> MSNVQTGAERMPHDLSHLGFLAGQIGRLITISTTPVIAGDSFEMDAVGALRLSPLRRGLAIDSTVDIFTFYVPHRHVYGEQWIKFMKDGVNAAPLPTVNTTGYIDHAAFLGTINPDTNKIPKHLFQGYLNIYNNYFKAPWMPDRTEANPNQLNEDDARYGFRCCHLKNIWTAPLPPETELSRQMTTSTTSIDIMGLQAAYANLHTDQERDYFMQRYRDVISSFGGKTSYDADNRPLLVMRSNFWASGYDVDGTDQTSLGQFSGRVQQTYKHSVPRFFVPEHGTMFTLALVRFPPTATKEIQYLNAKGALTYTDIAGD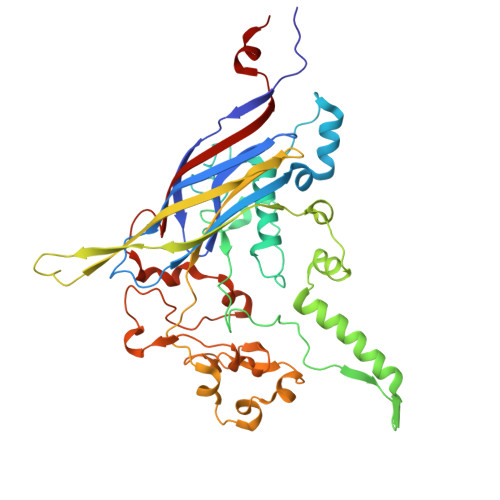PALYGNLPPREISMKDVFRSGDASKKFKIAEGQWYRYAPSYVSPAYHLLEGFPFIQEPPSGDLQERVLIRHHDYDQCFQSVQLLQWNSQVKFNVTVYRNLPTTRDSIMTS>MAHMKVYLDNNATTIVDPEVKAAMDPYFTQIYGNPNSLHDFGTECHPALRKAMDQMYEAIGARDEDDIVVTSCATESNNWVLKGVYFDLIKNGDKDHIITTEVEHPSVTATCRWLEEQGVRVTYLPVNQDGVVEAHTVRDFITDKTALVSIMWANNETGAIFPVEEISEICKEKGVLFHTDGVQAIGKIPVDVIRAGVDFMSFSAHKFHGPKGVGGLYIRNGHPLTSLLHGGEHMGGRRSGTLNVPGIVGMGKAMELA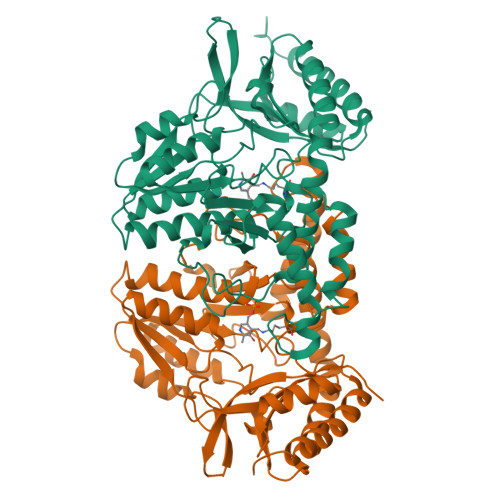TYYLKFEEEHVRKLRDKLEDAILEIPDTYSVGPRENRTPNTILVSVRGVEGEAMLWDLNRAGIAASTGSACASEDLEANPIMVAVGADSELAHTAVRLSLSRFTTEEEIDYTIEQFKKAVERLRSISSSYAYMPDNMKDKQLEVDLVPRGSHHHHHH[2x]>MNSSLPSLRDVFAN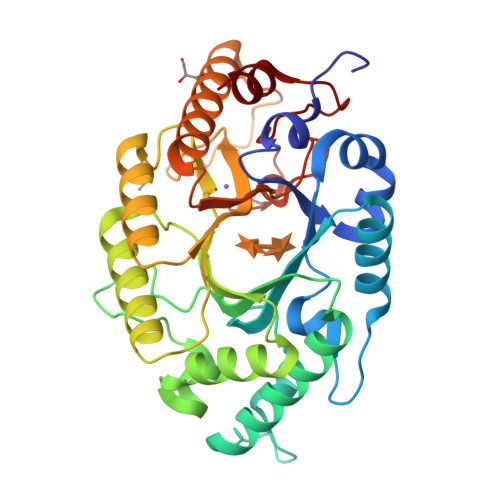DFRIGAAVNPVTIEMQKQLLIDHVNSITAENHMKFEHLQPEEGKFTFQEADRIVDFACSHRMAVRGHTLVWHNQTPDWVFQDGQGHFVSRDVLLERMKCHISTVVRRYKGKIYCWDVINEAVADEGNELLRPSKWRQIIGDDFMEQAFLYAYEADPDALLFYNDYNECFPEKREKIFALVKSLRDKGIPIHGIGMQAHWSLTRPSLDEIRAAIERYASLGVVLHITELDVSMFEFHDRRTDLAAPTSEMIERQAERYGQIFALFKEYRDVIQSVTFWGIADDHTWLDNFPVHGRKNWPLLFDEQHKPKPAFWRAVSV[2x]> MSRFVTSVSALAMLALAPAALSSGAYANDKLVELSKSDDNWVMPGKNYDSNNFSDLKQ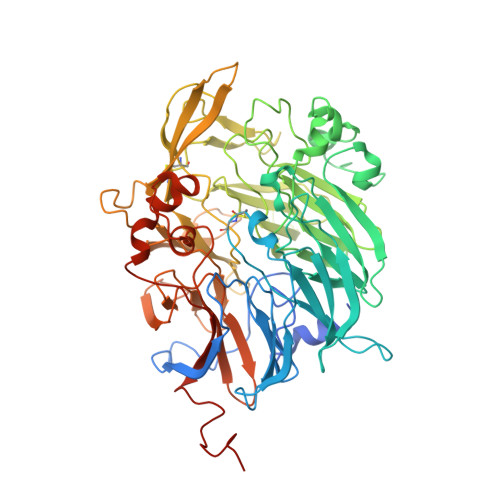INKGNVKQLRPAWTFSTGLLNGHEGAPLVVDGKMYIHTSFPNNTFALGLDDPGTILWQDKPKQNPAARAVACCDLVNRGLAYWPGDGKTPALILKTQLDGNVAALNAETGETVWKVENSDIKVGSTLTIAPYVVKDKVIIGSSGAELGVRGYLTAYDVKTGEQVWRAYATGPDKDLLLASDFNIKNPHYGQKGLGTGTWEGDAWKIGGGTNWGWYAYDPGTNLIYFGTGNPAPWNETMRPGDNKWTMTIFGRDADTGEAKFGYQKTPHDEWDYAGVNVMMLSEQKDKDGKARKLLTHPDRNGIVYTLDRTDGALVSANKLDDTVNVFKSVDLKTGQPVRDPEYGTRMDHLAKDICPSAMGYHNQGHDSYDPKRELFFMGINHICMDWEPFMLPYRAGQFFVGATLNMYPGPKGDRQNYEGLGQIKAYNAITGDYKWEKMERFAVWGGTMATAGDLVFYGTLDGYLKARDSDTGDLLWKFKIPSGAIGYPMTYTHKGTQYVAIYYGVGGWPGVGLVFDLADPTAGLGAVGAFKKLANYTQMGGGVVVFSLDGKGPYDDPNVGEWKSAAKHHHHHH Here we investigated the aminopeptidase, P. aeruginosa aminopeptidase (PaAP) from P. aeruginosa, which is highly abundant in the biofilm matrix. PaAP is associated with biofilm development and contributes to nutrient recycling. We confirmed that post-translational processing was required for activation and PaAP is a promiscuous aminopeptidase acting on unstructured regions of peptides and proteins. PaAP contains an M28 Zn peptidase domain (residues 44–116 and 274–510) and a PA domain (residues 117–273).

The PA domain was also captured in an alternative conformation in the truncated construct, PaAP_TE340A(trunc). These observations imply that the PA domain becomes free to rotate when not locked into an inactive conformation by the C-terminus interaction. Interestingly, the modified C-terminus (thrombin cleavage site, LVPR) is fully traceable in the PaAP_T structure and binds to the PA domain of an adjacent protomer, where the C-terminus interacts directly with R189A. The interaction of the C-terminus with an adjacent PA domain aids crystal packing, the protomers are linked together, akin to a chain. A similar observation was also seen in PaAP_TE340A(trunc), which instead packed head to tail. Autoprocessing was identified by comparing intact mass spectrometry results between active PaAP_T and inactive PaAP_TE340A, whereby a ten-amino-acid sequence is cleaved in PaAP_T. Interestingly, the thrombin-cleaved C-terminus of PaAP_TE340A (confirmed by intact MS) remained as a bound ligand in the crystal structure, suggesting that the liberated C-terminus propeptide is degraded by active PaAP.

>[6x]SEAQQFTEFWTPGKPNPSICKSPLLVSTPLGLPRCLQASNVVKRLQKLEDIASLNDGNRAAATPGYQASVDYVKQTLQKAGYKVSVQPFPFTAYYPKGPGSLSATVPQPVTYEWEKDFTYLSQTEAGDVTAKVVPVDLSLGAGNTSTSGCEAEDFANFPAGSIALIQRGTCNFEQKAENAAAAGAAGVIIFNQGNTDDRKGLENVTVGESYEGGIPVIFATYDNGVAWSQTPDLQLHLVVDVVRKKTETYNVVAETRRGNPNNVVMVGAHLDSVFEGPGINDNGSGSAAQLEMAVLLAKALPVNKVRFAWWGAAEAGLVGSTHYVQNLAPEEKKKIKAYLNFDMIGSPNFGNFIYDGDGSDFGLQGPPGSAAIERLFEAYFRLRGQQSEGTEIDFRSDYAEFFNSGIAFGGLFTGAEGLKTEEQAQKYGGTAGKAYDECYHSKCDGIANINQDALEIHSDAMAFVTSWLSLSTKVVDDEIAAAGQKLVPR> PNPCPESSASFLSRITFWWITGMMVQGYRQPLESTDLWSLNKEDTSEQVVPVLVKNWKKECAKSRKQPVKIVYSSKDPAKPKGSSKVDVNEEAEALIVKCPQKERDPSLFKVLYKTFGPYFLMSFLFKAVHDLMMFAGPEILKLLINFVNDKKAPEWQGYFYTALLFISACLQTLVLHQYFHICFVSGMRIKTAVIGAVYRKALVITNAARKSSTVGEIVNLMSVDAQRFMDLATYINMIWSAPLQVILALYLLWLNLGPSVLAGVAVMVLMVPLNAVMAMKTKTYQVAHMKSKDNRIKLMNEILNGIKVLKLYAWELAFKDKVLAIRQEELKVLKKSAYLAAVGTFTWVCTPFLVALSTFAVYVT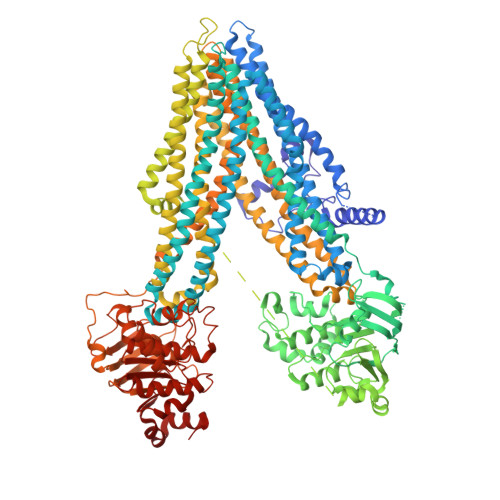VDENNILDAQKAFVSLALFNILRFPLNILPMVISSIVQASVSLKRLRVFLSHEDLDPDSIQRRPIKDAGATNSITVKNATFTWARNDPPTLHGITFSVPEGSLVAVVGQVGCGKSSLLSALLAEMDKVEGHVTVKGSVAYVPQQAWIQNISLRENILFGRQLQERYYKAVVEACALLPDLEILPSGDRTEIGEKGVNLSGGQKQRVSLARAVYCDSDVYLLDDPLSAVDAHVGKHIFENVIGPKGLLKNKTRLLVTHAISYLPQMDVIIVMSGGKISEMGSYQELLARDGAFAEFLRTYASAEQEQGQPEDGLAGVGGPGKEVKQMENGMLVTDTAGKQMQRQLSSSSSYSRDVSQHHTSTAELRKPGPTEETWKLVEADKAQTGQVKLSVYWDYMKAIGLFISFLSIFLFLCNHVASLVSNYWLSLWTDDPIVNGTQEHTQVRLSVYGALGISQGITVFGYSMAVSIGGIFASRRLHLDLLHNVLRSPISFFERTPSGNLVNRFSKELDTVDSMIPQVIKMFMGSLFNVIGACIIILLATPMAAVIIPPLGLIYFFVQRFYVASSRQLKRLESVSRSPVYSHFNETLLGVSVIRAFEEQERFIRQSDLKVDENQKAYYPSIVANRWLAVRLECVGNCIVLFASLFAVISRHSLSAGLVGLSVSYSLQVTTYLNWLVRMSSEMETNIVAVERLKEYSETEKEAPWQIQDMAPPKDWPQVGRVEFRDYGLRYREDLDLVLKHINVTIDGGEKVGIVGRTGAGKSSLTLGLFRIKESAEGEIIIDDINIAKIGLHDLRFKITIIPQDPVLFSGSLRMNLDPFSQYSDEEVWTSLELAHLKGFVSALPDKLNHECAEGGENLSVGQRQLVCLARALLRKTKILVLDEATAAVDLETDDLIQSTIRTQFDDCTVLTIAHRLNTIMDYTRVIVLDKGEIQEWGSPSDLLQQRGLFYSMAKDSGLV>[6x]GHMFFKDKNVLIIGGTGTIGKSILSNVLQEKPKVVRVFSRSEYNQFLLQEEFRDKNRN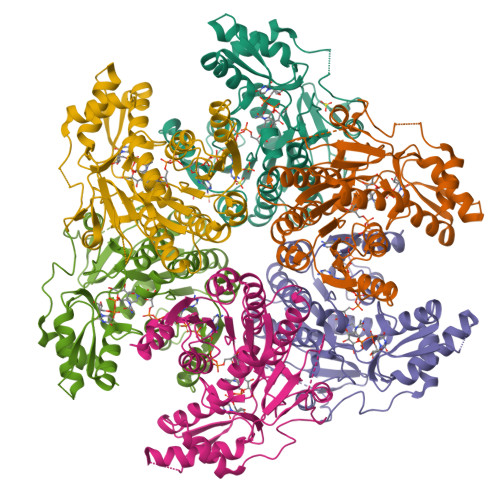IRYLIGDIRNYDRVFSAMENIDYVFHVAAMKHVSFCEYNPFEAVLTNIFGTQNVIKAAIAQKVKKVVFTSSNAAISPTNNYGATKLTAERLITSAEYSKGSSETTFTSVRFGNVMGSRGSVIPLFENQIKENQKITVTDLSMSRFMMTLNQATMLTIEAMKIAKGGETFILKMPVISLNDLSEVMIEEVTKLYGLSKENIKIEEIGLKPGEKMYEELMTHDESLQAFELPDMFIIPSPLKKGTQYENAKRAKAGFYRSDNQNAISKEELRNLILNQQLLTGGEKI> MVRESIPKEGENIKIQSYKHDGKIHRVWSETTILKGTDHVVIGGNDHTLVTESDGRTWITREPAIVYFHSEYWFNVICMFREDGIYYYCNLSSPFVCDEEALKYIDYDLD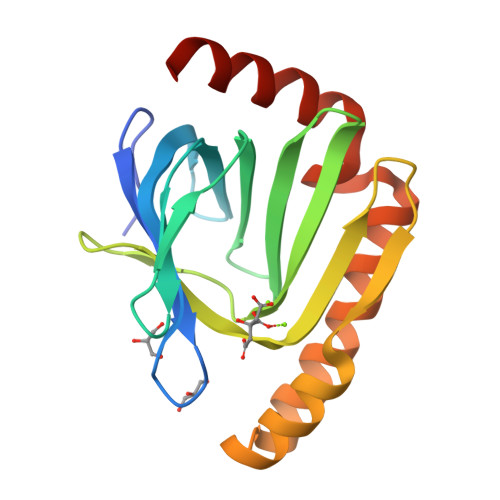IKVYPNGKYHLLDEDEYEQHMNQMNYPHDIDIILRRNVDILQQWIEQKKGPFAPDFIKVWKERYKKIRQY>M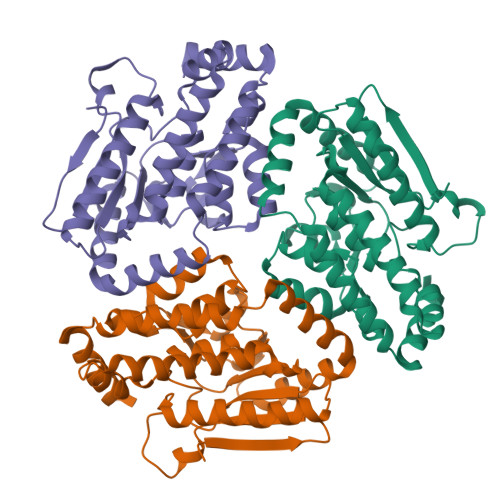GSSHHHHHHSQDPNSMSAVRPIITRPSQHPTLRITEEPERDVYWIHMHANLVNQPGRPCFASRLVDDIVDYQRELGDRLSASHALSPHVVLASDSDVFNLGGDLELFCRLIREGDRARLLDYAQRCVRGVHAFHAGLGTRAHSIALVQGNALGGGFEAALSCHTIVAEEGVLMGLPEVLFDLFPGMGAYSFLCQRISPRLAEKIMLEGNLYTASQLKEMGLVDIVVPVGEGVAAVEQVIKESRRIPHAWAAMREVNEIATMVPLHEMMRITEIWVDTAMQLGEKSLRTMDRLVRAQARRNGDPA[6x]> XVLK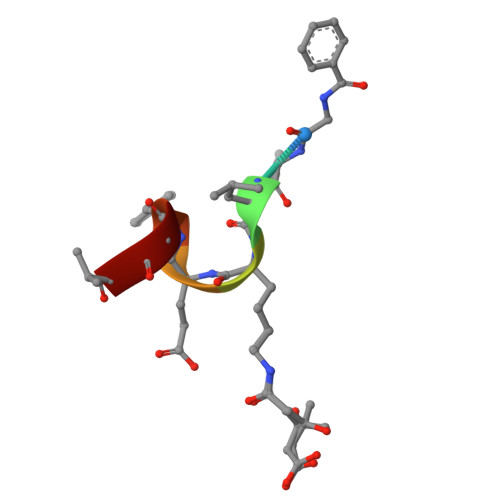EYGV> CSVPIQCT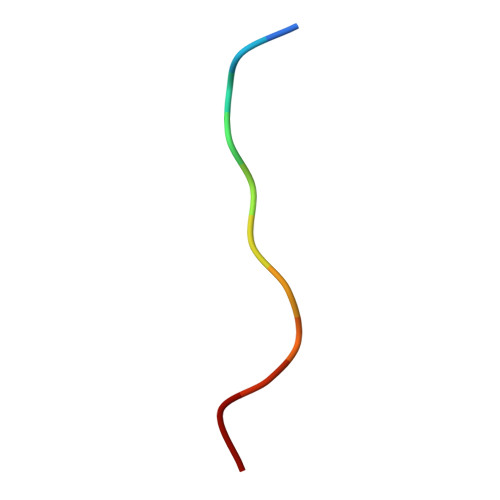DKT(3R,4R)-1-[3-amino-6-(3,4,5-trimethoxyphenyl)pyrazin-2-yl]-3-ethylpiperidine-4-carboxylic 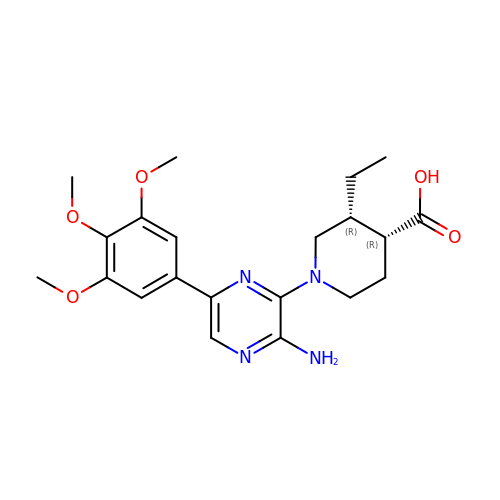acid | C21 H28 N4 O5 | MQOJTCBESRAKQA-GXTWGEPZSA-N> METDLNSQDRKDLD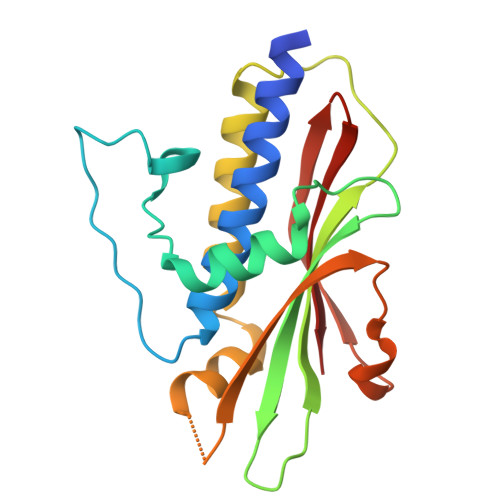KFIKFFALKTVQVIVQARLGEKICTRSSSSPTGSDWFNLAIKDIPEVTHEAKKALAGQLPAVGRSMCVEISLKTSEGDSMELEIWCLEMNEKCDKEIKVSYTVYNRLSLLLKSLLAITRVTPAYRLSRKQGHEYVILYRIYFGEVQLSGLGEGFQTVRVGTVGTPVGTITLSCAYR> GAEIPKEMLRAQTNYILLNVLKQGDNYVYGIIKQVKEASNGEMELNEATLYTIFDRLEQDGIISSYWGDESQGGRR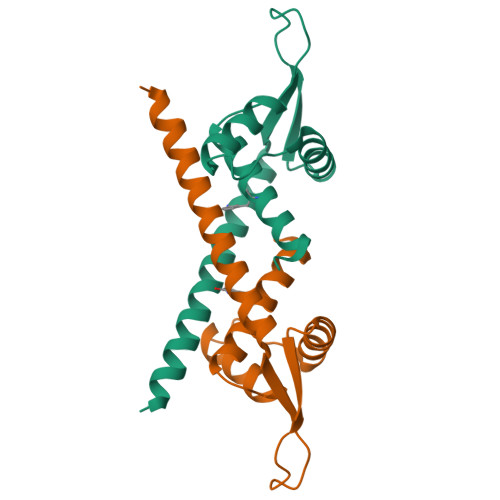KYYRLTEIGHENMRLAFESWSRVDKIIENLEANKKSEAIKSRGGSGGWSHPQFEK>[2x]SMPSQMEHAMETMMFTFHKFAGDKGYLTKEDLRVLMEKEFPGFLENQKDPLAVDKIMKDLDQCRDGKVGFQSFFSLIAGLTIACNDYFVVHMK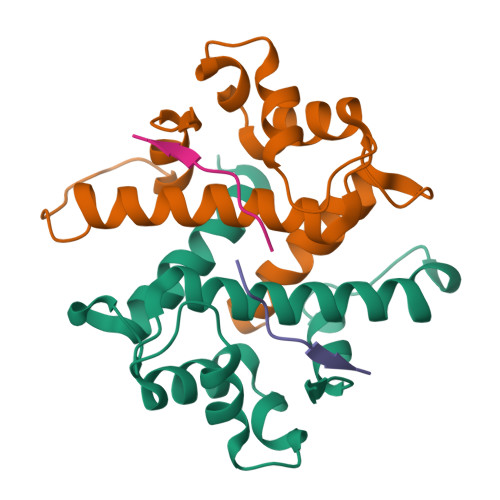QENLYFQGDSTVHEILSKLSLE;>[2x]QKVTFPKMKIPKFTF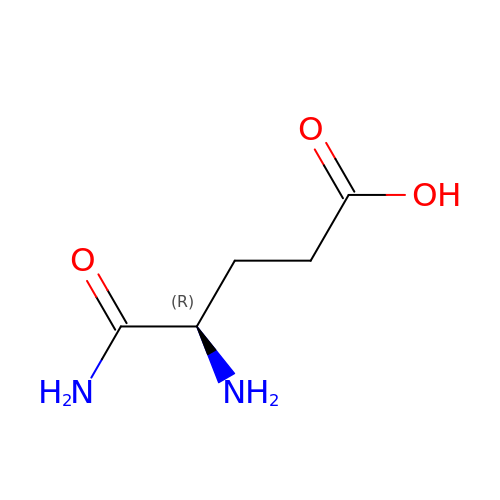D-alpha-glutamine | C5 H10 N2 O3 | AEFLONBTGZFSGQ-GSVOUGTGSA-N>[5x]MNDHIHRVPALTEEEIDSVAIKTFERYALPSSSSVKRKGKGVTILWFRNDLRVLDNDALYKAWSSSDTILPVYCLDPRLFHTTHFFNFPKTGALRGGFLMECLVDLRKNLMKRGLNLLIRSGKPEEILPSLAKDFGARTVFAHKETCSEEVD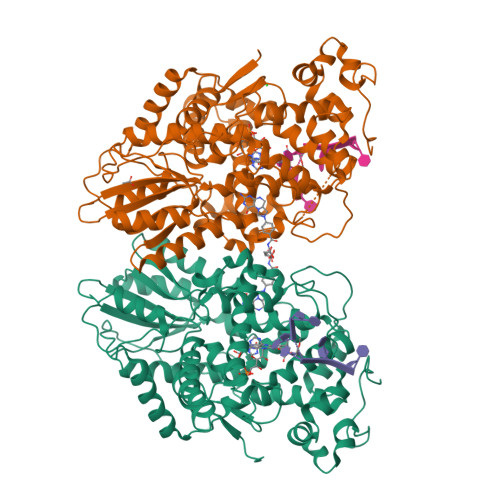VERLVNQGLKRVGNSTKLELIWGSTMYHKDDLPFDVFDLPDVYTQFRKSVEAKCSIRSSTRIPLSLGPTPSVDDWGDVPTLEKLGVEPQEVTRGMRFVGGESAGVGRVFEYFWKKDLLKVYKETRNGMLGPDYSTKFSPWLAFGCISPRFIYEEVQRYEKERVANNSTYWVLFELIWRDYFRFLSIKCGNSLFHLGGPRNVQGKWSQDQKLFESWRDAKTGYPLIDANMKELSTTGFMSNRGRQIVCSFLVRDMGLDWRMGAEWFETCLLDYDPCSNYGNWTYGAGVGNDPREDRYFSIPKQAQNYDPEGEYVAFWLQQLRRLPKEKRHWPGRLMYMDTVVPLKHGNGPMAGGSKSGGGFRGSHSGRRSRHNGP;> MNDHIHRVPALTEEEIDSVAIKTFERYALPSSSSVKRKGKGVTILWFRNDLRVLDNDALYKAWSSSDTILPVYCLDPRLFHTTHFFNFPKTGALRGGFLMECLVDLRKNLMKRGLNLLIRSGKPEEILPSLAKDFGARTVFAHKETCSEEVDVERLVNQGLKRVGNSTKLELIWGSTMYHKDDLPFDVFDLPDVYTQFRKSVEAKCSIRSSTRIPLSLGPTPSVDDWGDVPTLEKLGVEPQEVTRGMRFVGGESAGVGRVFEYFWKKDLLKVYKETRNGMLGPDYSTKFSPWLAFGCISPRFIYEEVQRYEKERVANNSTYWVLFELIWRDYFRFLSIKCGNSLFHLGGPRNVNGKWSQDQKLFESWRDAKTGYPLIDANMKELSTTGFMSNRGRQIVCSFLVRDMGLDWRMGAEWFETCLLDYDPCSNYGNWTYGAGVNDPREDRYFSIPKQAQNYDPEGEYVAFWLQQLRRLPKEKRHWPGRLMYMDTVVPLKHGNGPMAGGSKSGGGFRGSHSGRRSRHNGP> MHQQHSKSENKPQQQRKKFEGPKREAILDLAKYKDSKIRVKLMGGKLVIGVLKGYDQLMNLVLDDTVEYMSNPDDENNTELISK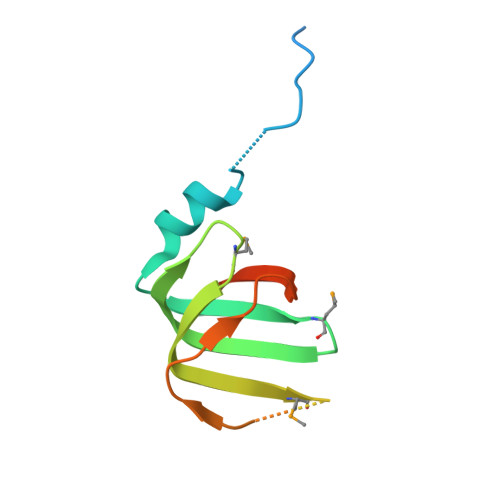NARKLGLTVIRGTILVSLSSAEGSDVLYMQK> MDKINLVCGSLLHNIGKIIYRGTSERAKHSKLGGDFIKSFEQFRNTELTDCIRYHHAQEITSVKSNKEKNSLFYITYIADNISSGMDRRKDLEEGAEGFNWDKKVALGSVFNVLNEKEKGRQNYSYPFVARTRIK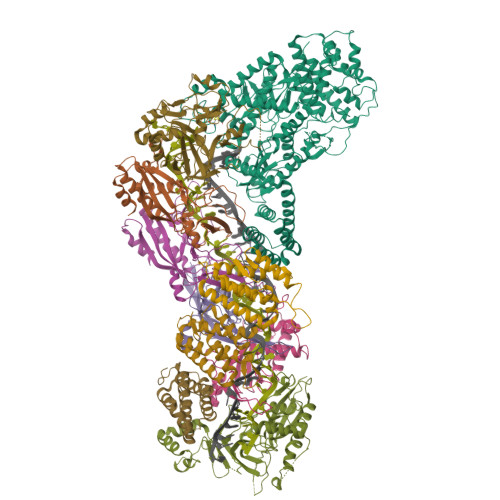EEPLNFPTATQNQYTTSYYDGLITDMKTILQRLKPDKEHINSLLQMMESLWSYVPSSTDKNQLVDISLYDHSRTTAAIASAIYDYFQAENITDYQKELFDYNATEFYDKNAFLMMNFDMSGVQNFIYNISGSKALKSLRARSFYLDMLLEYISDNLLEKLELSRANILYVGGGHAYLLLANTNKTKAILSDFEHDLKTWFLDKFKIDLYVAMAYTEVSANDLMNHNGHYRDIYRRLSQKTSAKKANRYTAEEILNLNHQGTENARECRECKRSDLLIEEDDICEICDSLQKVSRDLTRENIFVIANEGVLDMPFGKKMSALSYSQADKLKKSNAEVQIYAKNISEIGQNLMTRIDMGDYTYRSDFHEMLEEVEVGINRLGVLRADVDNLGQAFINGIPDDYLSISRTATFSRAMSRFFKNYLNQLLAEKSYKINVIYAGGDDLFMIGAWQDILDFSIVLKQKFADFTQNKLSISAGIGMFREKYPVARMASLTGDLEDAAKDYKPDERAVQATKNAVTLFDATNVFSWDTLENDIFVKLDAITKNFEKLDETGKAFIYRLIDLLRGVNENQQINIARLAYTLSRMEEKIGKTFAQELYNWANADRKTLIMALEIYILKTRE;> MKIIKLYFESPVHFGEKRLSESKITFSADTLFSALMIEAVGLGKEDEFYQLASNNLVKFSDAFPFIDQYYYIPKPMFNLKLEKEDENPSKAFKKLLYVPIDSLEDYLSGGLDAYFERESFNLGKLALSEKVQQHDFKDSEPYNVGTFTFKENTGLYVLIEQTHPLLEELLENLQYSGIGGKRNSGYGKFKFEILEDSDIEDLFSAKGNRKILLSGALPKDAELEQALKNASYLLERRGGFVQSDTYATNLVKKQDLYVFKSGSTFENSFDGDIYQVGKKGNHPVYKYAKSFFLEVS;>[3x]TELKIGNEKVNSTNFGDFAEKAIRGINHKPFVNSKGGEQKITTSKIRGILELVNKVYNRVINTNDVELSENILADIAYIKVKIAYESGREPVVKDFIQRTAFTAAITDVMNQRTRESFLLFARYVESLIAYFKFYGGKD;>[4x]MKLVIEGTIVLKTGMHIGGSSDFSAIGAVASPVVRDTLTRLPLIPGSSLKGKMRYLLAKELNNGILLNEPNNDQDEILRLFGSSEKDKIRRARLKFNDIKLSNLAELETFNVSSTEVKFENTINRKTAVANPRQIERVIAGSKFDFEIFYNLDDIKEVEKDFENIKQGFDLLEFDYLGGHGTRGSGRIAFENLSVITAVGNFEKINTLNEILGA;> MKKTYRVTLTALGPIFIGGGEKLKKYEYIFDKQKKVAHMIDHTKFTKYLLEKNLLDDFTSRVNSHFDLYDYLVNKKGIVFMPLVKYSVPVAQFRTEVKNRFGKPISSPPMNDLNTFVKDAFGRPYIPGSSLKGALRTAILNDLKEDTKENEVFAHLQVSDSETIDLENLKVYQKVDYSKTAKPLPLYRECLKPNTEITFTVSFDDEYLTLKKIQNALHKTYQHYYIKWLKGGKVGETLIKGVYDSHADELKKNTFALDQPSQNQGEIIYIGGGAGFVSKTLHYKSKNRDQARNDSFDILKQLFRTTYSKMRSVPDNVPVALKLAVETKTFNGRVTGKHYLEMGKARIKLEEL MamA is a magnetosome-associated protein (MAP) involved in the biomineralisation process by coating the magnetosome membrane. Each TPR consists of a helix-turn-helix fold, in addition to a putative N-terminal repeat. As such, MamA adopts an overall superhelical structure enabling the protein to be highly involved in protein-protein interactions via two main binding sites, one at its concave surface and the other at its convex surface.

Here, we have solved a new structure for MamA from the alternative species, Desulfovibrio magneticus strain RS-1, and compare between other, previously solved MamA structures and this distantly related species of MTB. By comparing these volumes to a standard calibration curve we determined that the three peaks correspond to sizes of a 13-meric oligomer, an octamer and a monomer. Crystallisation trials of octameric and monomeric ArsTM resulted in the appearance of a single crystal form that diffracted to a resolution of 2.88 Å (see Table 1 for data collection and refinement statistics). ArsTM monomers assemble to form a trimeric ring, each enclosing a ~15 Å diameter inner void; the crystal asymmetric unit includes six ArsTM monomers arranged as two trimeric rings. The employed forces that allow the stabilisation of each trimeric ring include salt bridges as well as hydrophobic interactions between the N-terminal of a single monomer and the C-terminal of a nearby monomer in a continuous manner, resulting in a ring with surface properties akin to a Möbius strip. As such, ArsTM presents a distinctly atypical binding surface since, as mentioned, the protein-protein interactions involving MamA typically bind via the concave or convex surfaces. Unexpectedly, but not altogether unsurprisingly, the triple mutated residues (E140A, K141A and E143A), along the ‘backbone’ of the monomers, were found to be at the centre of a crystal contact. The tight packing of ArsTM within the crystal could not occur with the original residues, which contained long and charged side chains and hence, could not be crystallised. The overall structure of the ArsTM monomer contains 10 anti-parallel α-helices, folded as five TPR helix-turn-helix motifs, namely TPR1 (H1 and H2), TPR2 (H3 and H4), TPR3 (H5 and H6), TPR4 (H7 and H8) and TPR5 (H9 and H10), similar to previously determined MamA structures. In ArsTM we could not detect such domain movement, as the conformations of all six monomers are similar. Whilst these salt bridge-forming residues are conserved in ArsTM (Arg47 and Asp76), the salt bridge itself is not since the distance between these two residues is too great.

>[6x]MAMGDKAKLYRNISQRCLRRGSPEEALRYLKEWARHEKNDPEPLYQMGIALANLGDYQRAVTVFDKVLKLRPNHFMASYRKGAVLLKIKQYKLALPVLEAVVAAAPADARAYYLLGLAYDGDEQLEKGIEAMQKAVDLDPEEIKYHQHLGFMNVRKDDHKTAAEHFTKVMELERSQDSDEEELALVPRGSSAHHHHHHHHHH> MRDIVFVSPQLYLSSQEGWKSDSAKSGFIPILKNDLQRFQDSLKHIVDARNSLSETLLNSNDDGSIHNSDQNTGLNKDKEASIADNNSANKCATSSSRYQELKQFLPISLDQQIHTVSLQGVSSSFSRGQIESLLDHCLNLALTETQSNSALKVEAWSSFSSFLDTQDIFIRFSKVDEDEAFVNTLNYCKALFAFIRKLHEDFKIELHLDLNTKEYVEDRTGTIPSVKPEKASEFYSVFKNIEDQTDERNSKKEQLDDSSTQYKVDTNTLSDLPSDALDQLCKDIIEFRTKVVSIEKEKKMKSTYEESRRQRHQMQKVFDQIRKNHSGAKGSANTEEEDTNMEDEDEEDDTEDDLALEKRKEERDLEESNRRYEDMLHQLHSNTEPKIKSIRADIMSAENYEEHLEKNRSLYLKELLHLANDVHYDHHRSFKEQEERRDEEDRAKNGNAKELAPIQLSDGKAISAGKAAAITLPEGTVKSENYNADKNVSESSEHVKIKFDFKKAIDHSVESSSEDEGYRESELPPTKPSERSAAEDRLPFTADELNIRLTNLKESRYVDELVREFLGVYEDELVEYILENIRVNQSKQALLNELRETFDEDGET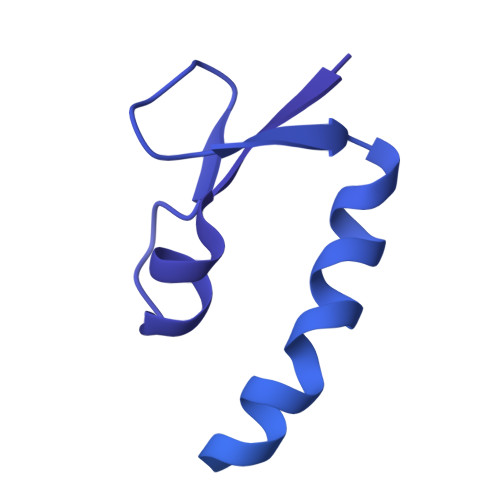IADRLWSRKEFRLG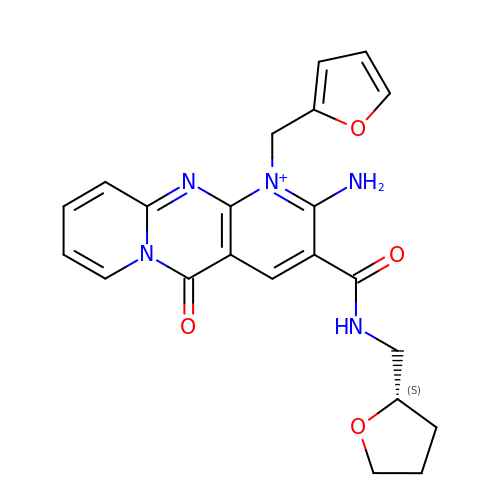2-amino-1-[(furan-2-yl)methyl]-5-oxo-3-({[(2S)-oxolan-2-yl]methyl}carbamoyl)-5H-dipyrido[1,2-a:2',3'-d]pyrimidin-1-ium | C22 H22 N5 O4 | KUXUMXOWEWRGNF-AWEZNQCLSA-O On the other hand, U2AF small subunit, U2AF1, binds to the 3′ side of the boundary sequence between the exon and intron, known as the 3′ splice site (3′SS). Then, the recognition of 3′SS by U2AF1 is a critical step for the determination of the excluded intron for the production of mature mRNA. U2AF1 consists of conserved three domains, an N-terminal zinc finger (ZF1), a U2AF homology motif (UHM), and a C-terminal zinc finger (ZF2). As U2AF1 was stabilized by the binding of U2AF223, structural and biochemical experiments were carried out with a complex of Schizosaccharomyces pombe U2AF1 with the short fragment of U2AF2 spanning residues 93–161 (the U2AF1 complex), as previously reported.

In order to clarify where and how U2AF1 binds to RNA, we solved the crystal structure of U2AF1 complex with RNA containing 3′SS sequence, 5′-UAGGU. Nine copies of the U2AF1 complex with RNA are found in the asymmetric unit. Without RNA, N-terminal 14 amino-acid residues are disordered and not visible in the electron density. This region of U2AF1 is stabilized by interaction with RNA, and ten additional amino-acid residues (Leu5–Lys15) can be modeled in the RNA-bound form. The −2A base is stacked by the aromatic ring of Phe20, and is sandwiched by the side chain of Arg28 in ZF1. The nearby Cys27, which coordinates a zinc ion, accepts a hydrogen bond from the N6-amino group of the adenine −2A. On the other hand, the side chain of Phe165 (in ZF2) interacts with the guanine bases at positions −1 and +1 through perpendicular and parallel π–π stacking, respectively. The O4-carbonyl oxygen of −3U forms a hydrogen bond with the main-chain amide proton of Ser34, whose hydroxyl side-chain hydrogen bonds to N3 imino proton of –3U. Our present crystal structure indicates that U2AF1 has a strong preference for guanine at the +1 position in the exon sequence. +1 G forms a π–π interaction with Phe165 and cation–π interaction with Arg150 involves the six-membered ring of the base, which lies further from the RNA backbone than the five-membered ring.

>[9x]MASHLASIYGTEQDKVNCSFYYKIGACRHGERCSRKHVKPNFSQTILCPNMYKNPIHEPNGKKFTQRELAEQFDAFYEDMFCEFSKYGEVEQLVVCDNVGDHLVGNVYVRFKYEESAQNAIDDLNSRWYSQRPVYAELSPVTDFREACCRQHETSECQRGGLCNFMHAKKPSPQLLRDLVLAQRKYLALNAAEEMKKEPNSDSTNRWVSVTAERKN;>SSVGRSRSPPPSRERSVRSIEQELEQLRDVTPINQWKRKRSLWDIKPPGYELVTADQAKMSGVFPLPGA[9x]>MGSSHHHHHHSQDPENLYFQSMSPKDLTIPTGADGEGSVQVHLDEADKITGAKVFAVYGKGGIGKSTTSSNLSAAFSILGKRVLQIGCDPKHDSTFTLTGSLVPT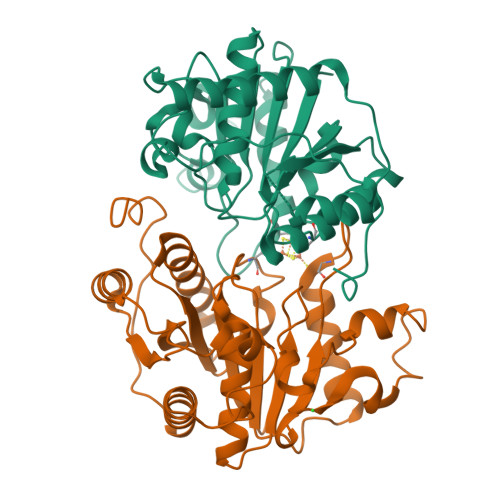VIDVLKDVDFHPEELRPEDFVFEGFNGVMCVEAGGPPAGTGCGGYVVGQTVKLLKQHHLLDDTDVVIFDVLGDVVCGGFAAPLQHADQAVVVTANDFDSIYAMNRIIAAVQAKSKNYKVRLAGCVANRSRATDEVDRFCKETNFRRLAHMPDLDAIRRSRLKKKTLFEMDEDQDVLAARAEYIRLAESLWRGLDPIDPHSLPDREIFELLGFD[4x]> MSLRPCFVSLIDESDKPILIYVPNEAENEMNDVLKYNVLSNISLDYFESALVEWHSLDSKPLLKSIFQLEGVSVFAMLIKQTGLKIVIGFEQKSLSGADDEFEAINQIFETVRKIYIRVKCNPLLVSGDEKSIIKSLERKFDELFISTEVEL;> MSSTHSNNVGHPQSSPQGPLTEQQRAQQQYQIFENSLPKVSQSVYQMLLNEMVPLAMGIERQISGDVISSDSNVTSENGNINNMIKRLKIEEHHTVDIIRSHNLIHELYKADEEEKEKVLARLRNIGFQIGLKLSELLIFSNNPNLKFKEMDLLLIMKFICRDVWKQIFGKQIDNLKTNHRGTFYLLDYDYRPIQSFSLEEDAKNEELKMIEPFLEIPVGIIRGVLSSLGYSSEEVICLASFIDRPTDRPKTAFPKGVSFHVQVTMPQ;>MVSTTQSRSLKAMGEEIWKNKTEKINTELFTLTYGSIVAQLCQDYERDFNKVNDHLYSMGYNIGCRLIEDFLARTALPRCENLVKTSEVLSKCAFKIFLNITPNITNWSHNKDTFSLILDENPLADFVELPMDAMKSLWYSNILCGVLKGSLEMVQLDCDVWFVSDILRGDSQTEIKVKLNRILKDEIPIGED[2x];> MGIYSFWIFDRHCNCIFDREWTLASNSASGTINSKQNEEDAKLLYGMIFSLRSITQKLSKGSVKNDIRSISTGKYRVHTYCTASGLWFVLLSDFKQQSYTQVLQYIYSHIYVKYVSNNLLSPYDFAENENEMRGQGTRKITNRNFISVLESFLAPMVNQ;> MAIETILVINKSGGLIYQRNFTNDEQKLNSNEYLILASTLHGVFAIASQLTPKALQLTQQTNIENTIPYIPYVGMSSNRSDTRNGGGNNNKHTNNEKLGSFKGDDFFKEPFTNWNKSGLRQLCTDQFTMFIYQTLTGLKFVAISSSVMPQRQPTIATTDKPDRPKSTSNLAIQIADNFLRKVYCLYSDYVMKDPSYSMEMPIRSNLFDEKVKKMVENLQ;> MSQRIIQPSASDQQFPGKSDGYEYTVGPKQAITSEASTTYIPSRIYSESLLFKRQEASLSAMAFLFQEMISQLHRTCKTAGDFETKLSDYGHNIGIRLLELLNFRASSSPSSLPRASAFLSQNESSSKLSNASNSPGMLANSSTATSASANERLQEKQTESLSNYITKMRRRDLKILDILQFIHGTLWSYLFNHVSDDLVKSSERDNEYMIVDNFPTLTQFIPGENVSCEYFVCGIIKGFLFNAGFPCGVTAHRMPQGGHSQRTVYLIQFDRQVLDREGLRFG;> MPQYFAIIGKKDNPVYEIEFTNAENPQGFPQDLKELNPFILHASLDIVEDLQWQINPTSQLNGNGGNGSNGGGGFLRSRAVNNTDNCYLGKVDHFYGLAITAYISYSGMKFVMIHGNSANSSVVIDDNNMRSFYQEVHELYVKTLMNPFYKITDPIRSPAFDSRVRTLARK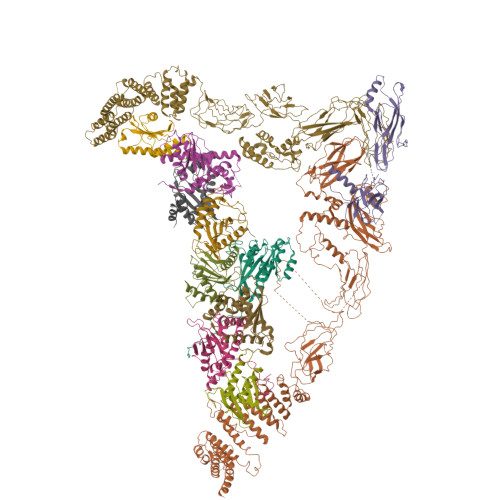HLSK;> MDKEIYCGSVPVSYFDPFDLFESLRPEFQQILPLDNIHWKAFDGTVRTVNRLPIELIPEGRGEADKSNDEQPFIRFLIVNCISIDQYRAKVRPLVRQWLPNLESVSSSTGEKMIYKPIILLYANSEVVDSNLFKSVSLMEKFGKDFPHVQTLEVRSVYRSPKERQEFWNQFSQKIKASVLSIFQKRLTHLQHSLANLQKGNNFEEQLLTREKLYELYVVFNILEDASLELQKIKKEILRRNMNMPDGKLQVPFESSSKSDESLGSIIIEGTLDKFQLHKYFFIRRLRLLKLEDQTLTAFVGAFQLIKNFIESISIEYRKSVRLLEFKHYFITSMLSYFEFENVSNPLLCEIKAELLMLKRDNWVQGVMATSGYRLMDKNYPNSDVKYKFDLLKETFVDETVFQENFLTLTKEILSLFNKCEGKRQRIVDILSIEIGLLYYQGKKYEEAVSLFLSCYEYYTQTNKNSIGLKILQVFIDSLSHCPKLDVLQIDGESVSASAVLTNAFLNILKLCKDNDSKEIWWKKFMDLQMKNNIHLMYPLDGLFEVTLNSKVHLARANVSAIEVNLKSYGFPEDISTKTMRLSLKNMGGDVIVFGASDFLLKKGENKLILECRDIMYGEFSLLSFEIIVEGITFVKEFPENQDEFIVVPEIYCKESTKVLVKQAHNLNLGEYALELKSVQSDALESLQVEVEVQKNIGNMKNLPVSFSMDEIQARKRYNTPFENVRLEYYLLDQITAFDLIIKTSFTKKNDQGTFGETKKVRIQCYLQLSVSVEDIFKKDIFFFKFLLNSSVREEPVILYSSELSAPDTRNDYNIRGDYIATTPALITFDGNESFINCYEITANNNFDSKDIFNLKVRYNTLKEQLDCFITDAVLIEGDVEWFILFEKWKTFWELEILKKLKYDYDAFKENRIIRLLKTSIDLNKTKSKIRNLCIEKAVLDKILICLNKVSRGIAVCNTDMDEYVRNLVPKQLTVPVQLPGFEQFFHVQFEQMETSHDALHDTIATIGNSLSYTVIVENLSGQWGQDVIDDGGYIFEILSSNEWLIHGQKRCAIKEKRKEFEVHLIPLKKGYLNFPRVEITNINGKSCRVDHSNAFESILIF;> MNILKHFPSYVGPSKIRTLVIPIGHWTRKEFNNAVQKLSEFNEIHLSDVTPIDSPIFTPQGFPHGKLFFDFLTIDHDDALELFLYDFEPFRKTFVIIGLVNDYSDPLTNLNFMKEKYPTLISPNLVYASSTPTKELEQTIDTMENVFASSPDMQKNIETIMCDIARNFLTALNSYYSSYKHVTLRSPGAIGGNAVLKTTLIRQNSYTSSSSSTPMSAVQSSVSSSSKAGSVTTASKRLSSFEMTTNSLKRSASLKLATTLSTSENRSQQKSLGRQMKILGNFQLLAGRYVDALNSFVDAITTLYKVRDYLWLGSALDGISICFLLLSYLGLSYQIPQIVSLICPVEKLNFESSSTGISPVDSNSKATASTTASSTPRNSISIAAMQSPRNSIMSLSAPALNIDVENINLPLLIKCISDKVLYYYDLSLMHNSEYAPQVVYCEFLLKTLTFMTSCYKSSEFSKDVLDNIVKNQHRALSDIPNSPMFPRFEVYFYSNKLFELQLKEMQVEAQIKIYSTMAEVYRLLGYKRKQLFVLRLLMVALLATPNKIAWHPDYRTLIDTIIELLNINESEAKINVDDPSQSTWLILQKKILQLCIKVSRKINDFEYVAKFSSILITKYTHLLNQSEQDALFKEYIQPSITNESITSYWDPFILREVVINRILDSDPTSNEIPLESDVSSLESLENRQKTQDINPQEVFNPFKRVQPTSFVSNNSTKVPILVFLVGDKAEFTCRVQNPFKFDFTINDIQLDEEISEFCEIDRKAVSYSGPYNVKAESIRSITLPLIIKKPTYKKIYEISCLKISILKLPLQKFDIINDSRRSNPVEEEAEYSKCIYGKLKIKILPEQPQLELLSTSKMTRNSWMMLDGTKTDFHITVRNKSLSCAINHIKIIPMNNIEQMLKPDYWKKMPPDDLYIMEKQLDWLSKSCVRIIKLPTVIKPNETITFDLELDNTAVPFNFTGFDLLIEYGMSATDESCIYLKKLSIPYEVTLRRTIEVPSMDIIPLNELFSSQVENVDWIEYVMSKIRAESNLHSRDFILLLLDFRNSWIDGIKLNVQFEDFTSNEYHVEASHTSRIIVPIKKIDYKKYNFENTPIPRIYPGRQFIQSGLNEEQTIEMRQKFWCREHIISKLKCNWKLTTDQSVTGSVDFNKFIEKFDHKMVYTIYPGRLFYGVQLLLDEPKVKVGEIINLKIITEPTSTCRRKQNSTVNFLDIVIFDSKTSKILPRSNRRILYNGSLTKPISTTKVSEINLEIIPIEKGRYEFSVCISKSNNQDGIIQFDSENVILSVI;> MECFVPLRCDLDGSNIEQLRQSHLSRKFIIFDEQLNLWLWFQGNSQENKRFVLQNMIILINEAQVTRTSTIDDYFTQVENNENLWRLKNDCCSKILFKSNVVMNNGYNNQIKFVFEYKSVDANFNNQDSLQDPQAKYTLDKYSSEEILPSFEPVYSWSSAATKSSKNTNNHLEKNNRATHRVSSKNSEVHEADVSRNPNTFTLKLQYPIFSLLNMRLRNISLKSEHCILSSLDFQTSKASEQLTKKFIYPQEHNSFLKLNFQEISYKLIDGTSQIELDPICPLKVPLTAFSYDSISATFKLVLLPKSTQPHRVKITLAYELELHPNLKLPVRTSWETEVTLKRSMPISSTSSQYSSNNNNTNHSASFNGAANNVNSGGLANLRLGGVSSSRFSLGAASTTSLVNSKLSNVKFKFINSNIKVIKGEKFTMRLQIINSSSSPLDLVVYYNNTINPIPSANNVRNSNGINNCGMNNGTIPNSPLTLENQYQLHNKYRKIAEGIILLSNDYKIPVVPPRETYFADLRFIGIMSGYYGTLSGLKVLDLNTNELIEVGNGASVLIQ;> MSNEDYGYDYDYLFKIVLIGDSGVGKSNLLSRFTTDEFNIESKSTIGVEFATRTIEVENKKIKAQIWDTAGQERYRAITSAYYRGAVGALIVYDISKSSSYENCNHWLTELRENADDNVAVGLIGNKSDLAHLRAVPTDEAKNFAMENQMLFTETSALNSDNVDKAFRELIVAIFQMVSKHQVDLSGSGTNNMGSNGAPKGPTISLTPAPKEDKKKKSSNCC>MSAFELKNLNDCLEKHLPPDELKEVKRILYGVEEDQTLELPTSAKDIAEQNGFDIKGYRFTAREEQTRKRRIVRVGAIQNSIVIPTTAPIEKQREAIWNKVKTMIKAAAEAGCNIVCTQEAWTMPFAFCTREKFPWCEFAEEAENGPTTKMLAELAKAYNMVIIHSILERDMEHGETIWNTAVVISNSGRYLGKHRKNHIPRVGDFNESTYYMEGNTGHPVFETEFGKLAVNICYGRHHPQNWMMFGLNGAEIVFNPSATIGRLSEPLWSIEARNAAIANSYFTVPINRVGTEQFPNEYTSGDGNKAHKEFGPFYGSSYVAAPDGSRTPSLSRDKDGLLVVELDLNLCRQVKDFWGFRMTQR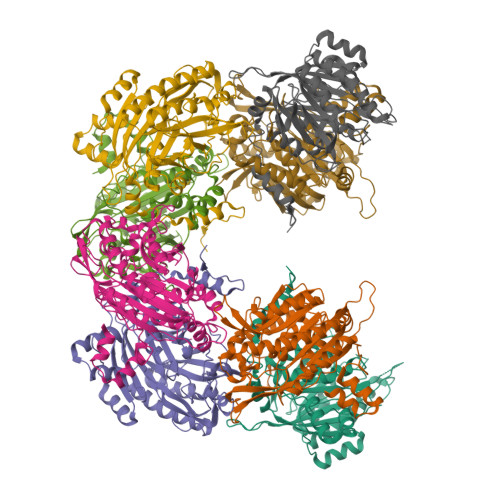VPLYAESFKKASEHGFKPQIIKETQFPGDDDDKHHHHHHHHSG[8x]> MHKINKWS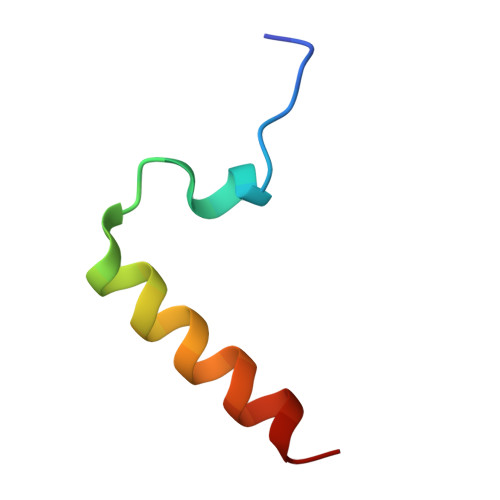VIYNINSTVTRALRDLMQGILQKI> EDVDECAMANSNPCEHAGKCVNTDGAFHCECLKGYAGPRCEMDINECHSDPCQNDATCLDKIGGFTCLCMPGFKGVHCELEINECQSNPCVNNGQCVDKVNRFQCLCPPGFTGPVCQIDGSGLEVLFQGPGSLHHILDAQKMVWNHRGHHHHHHHH

The Notch signalling pathway is conserved across all metazoan species and plays key roles in many aspects of cell biology including cell‐fate determination, stem cell maintenance, immune system activation and angiogenesis in humans (Guruharsha et al, 2012; Bray, 2016). Aberrant Notch signalling results in a number of inherited and acquired disorders, including various cancers, and it is therefore a key target for therapeutic intervention (Hansson et al, 2004; Groth & Fortini, 2012). Both the Notch receptors and the ligands are single‐pass type I transmembrane proteins, and direct protein–protein contact between adjacent cells initiates an intracellular signalling pathway. All of the Notch ligands have a modular extracellular architecture consisting of an N‐terminal C2 domain (formerly known as the MNNL domain), a Delta/Serrate/Lag‐2 (DSL) domain, and either 16 (Jagged1/Jagged2), 8 (Delta‐like1/Delta‐like4) or 7 (Delta‐like3) EGF repeats. Binding of a Notch ligand to EGF11‐12 of a Notch receptor results in a series of proteolytic cleavages, with the final intra‐membrane cleavage by gamma secretase, causing the release of the intracellular domain of Notch (NICD) from the plasma membrane.

We have also solved the structure of human Notch2 EGF11‐13, which includes the ligand‐binding region (EGF11‐12). Human Notch2 EGF11‐13 has 67% sequence identity with human Notch1, and superposition of the two structures shows that both adopt a very similar linear arrangement (RMSD = 1.55 Å). In our crystal structure, Notch2 is O‐fucosylated on Thr‐470, and O‐glycosylated on Ser‐462 and Ser‐500. In the earlier Notch1‐Delta‐like4 structure, the O‐fucose on the equivalent threonine residue in EGF12 is seen to be involved in direct intermolecular binding to the C2 domain (Taylor et al, 2014; Luca et al, 2015). In contrast, the O‐glucose modifications affecting specific serine residues in Notch2 appear to stabilize intramolecular structure as observed previously for the Notch1 complex (Luca et al, 2015): the disaccharide (glucose + xylose) on Ser‐462 may stabilize Notch2 EGF12 through interaction with Phe‐478 (shown), shielding it from the solvent. Similarly, the O‐glucose on Ser‐500 may stabilize EGF13 through interaction with Phe‐516. The availability of our new structures of hJagged2, hDelta‐like4 and hNotch2 allows modelling of the receptor‐binding interface across all canonical ligands and Notch1/Notch2 and show that almost all of the key residues involved in ligand binding (Leu‐468, Asp‐469 and Ile‐477 in site 1; Phe‐436 and Arg‐448 in site 2) are conserved in Notch2. All canonical human Notch ligands (Jagged1, Jagged2, Delta‐like1 and Delta‐like4) (N‐EGF3) bind to both human Notch1 (i) and Notch2 (ii) EGF11‐13 to a similar extent as assessed by plate assay.> MTAAVTPSASAVASDDKKSERRLAFWLIAPAVLLMLAVTAYPIGYAVWLSLQRYNLAEPHDTEFIGLANYVTVLTDGYWWTAFAVTLGITVVSVAIEFALGLALALVMHRTIFGKGAVRTAILIPYGIVTVAASYSWYYAWTPGTGYLANLLPEGSAPLTDQLPSLAIVVLAEVWKTTPFMALLLLAGLALVPQDLLNAAQVDGAGPWKRLTKVILPMIKPAILVALLFRTLDAFRIFDNIYILTGGSNDTGSVSILGYDNLFKAFNVGLGSAISVLIFLSVAIIAFIYIKIFGAAAPGSDEEVR;> MADRVDARRATWWSVVNILVIVYALIPVLWILSLSLKPTSSVKDGKLIPTEITFANYKAIFSGDAFTSALFNSIGIGLITTIIAVVIGGMAAYAVARLQFPGKQLLIGVALLIAMFPHISLVTPIFNMWRGIGLFDTWPGLIIPYITFALPLAIYTLSAFFREIPWDLEKAAKMDGATPAQAFRKVIAPLAAPGIVTAAILVFIFAWNDLLLALSLTATQRAITAPVAIANFTGSSQFEEPTGSIAAGAMVITIPIIIFVLIFQRRIVAGLTSGAVKG;>[2x]MAEIVLDRVTKSYPDGAGGVRAAVKEFSMTIADGEFIILVGPSGCGKSTTLNMIAGLEEITSGELRIGGERVNEKAPKDRDIAMVFQSYALYPHMTVRQNIAFPLTLAKVPKAEIAAKVEETAKILDLSELLDRKPGQLSGGQRQRVAMGRAIVRSPKAFLMDQPLSNLDAKLRVQMRAEISRLQDRLGTTTVYVTHDQTEAMTLGDRVVVMLAGEVQQIGTPDELYSSPANLFVAGFIGSPAMNFFPATRTDVGVRLPFGEVTLTPHMLDLLDKQARPENIIVGIRPEHIEDSALLDGYARIRALTFS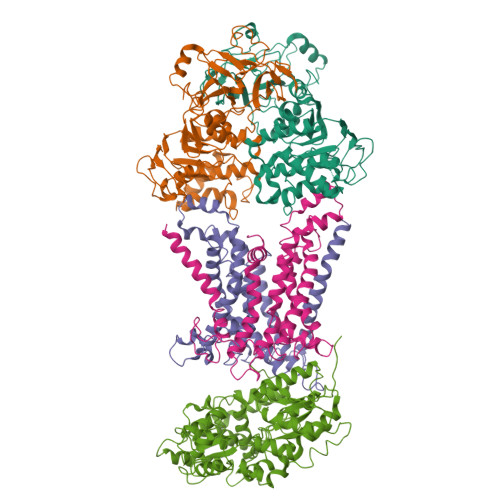VRADIVESLGADKYVHFTTEGAGAESAQLAELAADSGAGTNQFIARVSADSRVRTGEQIELAIDTTKLSIFDAATGLNLTRDITPTDPTEAAGPDAG;> MRARRLCAAAVAAMAAASMVSACGSQTGGIVINYYTPANEEATFKAVANRCNEQLGGRFQIAQRNLPKGADDQRLQLARRLTGNDKSLDVMALDVVWTAEFAEAGWAVPLSEDPAGLAEADATENTLPGPLETARWQDELYAAPITTNTQLLWYRADLMPAPPTTWDGMLDEANRLYREGGPSWIAVQGKQYEGMVVWFNTLLQSAGGQVLSDDGQRVTLTDTPEHRAATVKALRIIKSVATAPGADPSITQTDENTARLALEQGKAALEVNWPYVLPSLLENAVKGGVSFLPLDGDPALQGSINDVGTFSPTDEQFDIAFDASKKVFGFAPYPGVNPDEPARVTLGGLNLAVASTSQHKAEAFEAIRCLRNVENQRYTSIEGGLPAVRTSLYDDPAFQKKYPQYEIIRQQLTNAAVRPATPVYQAVSTRMSATLAPISDIDPERTADELTEAVQKAIDGKGLIP>APKAPADGLKMEATKQPVVFNHSTHKSVKCGDCHHPVNGKEDYRKCGTAGCHDSMDKKDKSAKGYYHVMHDKNTKFK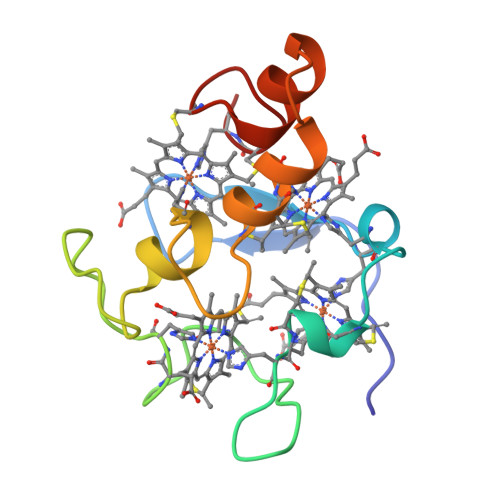SCVGCHVEVAGADAAKKKDLTGCKKSKCHE[2x]>MASWSHPQFEKGAMTARKVDYTDGATRCIGEFHWDEGKSGPRPGVVVFPEAFGLNDHAKERARRLADLGFAALAADMHGDAQVFDAASLSSTIQGYYGDRAHWRRRAQAALDALTAQPEVDGSKVAAIGFCFGGATCLELARTGAPLTAIVTFHGGLLPEMAGDAGRIQSSVLVCHGADDPLVQDETMKAVMDEFRRDKVDWQVLYLGNAVHSFTDPLAGSHGIPGLAYDATAEARSWTAMCNLFSELFG[2x]

A microfluidic screening platform is used to recover and identify various hydrolases from metagenomic sources by screening for the hydrolysis of two substrates: sulfate monoesters, containing one of the most unreactive functional groups in biology32, and phosphate triesters. The high sensitivity of our platform enabled us to isolate enzymes with strong and weak activities, including promiscuous side activities that have not been selected in the course of evolution and could not be predicted by sequence homology. Applying the screening workflow to PTEs (using triester 2d as substrate) led to the isolation of eight unique and novel sequences, mostly originating from unknown microorganisms. (iii) One hit, P91, is a member of the α/β-hydrolase (α/β) superfamily related to dienelactone hydrolases (DLHs).

Members of this superfamily possess a catalytic triad41, whereas most bacterial PTEs described to date use catalytic divalent ions to activate a water nucleophile42. The X-ray structure of the protein was determined at a resolution of 1.7 Å and structural alignment with a previously characterized DLH43 (also identified in the SSNs) confirmed an α/β hydrolase fold, and highlighted a homologous catalytic triad in the active site of P91 (C118, D167 and H199). Site-directed knockdown mutagenesis of C118, D167 and H199 led to enzyme inactivation, consistent with catalysis by the cysteine-based catalytic triad in P91, which was expected to provide nucleophilic and charge relay catalysis. We observed electron density consistent with two orientations of C118. Figure 5b highlights potential ‘protecting' residues (E37 and H141) that may play a role in stabilizing an inactive conformation of the nucleophile cysteine, as previously invoked44. The lack of electron density in the vicinity of the active site supported the absence of a metal-binding site, underlining a role for the triad instead of a metal cofactor in catalysis. Functional tests further ruled out P91 as a metallo-enzyme: treatment of P91 with chelating agents did not affect its activity towards triester 2a, whereas a reduction (or complete abolition) of activity was observed in all other PTE hits tested. However, P91 is the first metal-free bacterial (or archaeal) triesterase to be described, unrelated to insect carboxylesterases. The comparison of the Michaelis–Menten parameters (kcat/KM and KM) of our triesterase hits with those of (i) OP hydrolases isolated from pesticide-contaminated soils and (ii) enzymes with known promiscuous triesterase activity suggests that paraoxon 2a (or parathion 2b with lower or similar catalytic rates measured) and, by extension, the synthetic triester 2d are not the physiological substrates of our hits. This conclusion was also supported by the experimental verification of higher activities in P83, P84, P90 and P91 towards lactone 8c, thioester 7 and ester 6, respectively.5-N-acetyl-4-guanidino-6-methyl(propyl) carboxamide-4,5-dihydro-2H-pyran-2-carboxylic 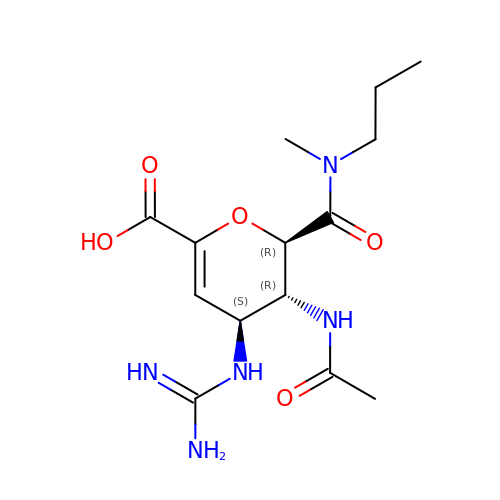acid | C14 H23 N5 O5 | QPJWMZVTNXFTKV-JMJZKYOTSA-N> MHYAEAATPAKSAGSAVAKKHLEAKQKIGFVHGIDGTIATIAPAASKVTVPYNTVLEIAVSATNIANALVFNLEKDGSIGVILLDNISEVRSGQDVYATGSLLKIPVGFHMLGKIINPLGKEIPTGLFTKAAPLLDDTKLGLVEEMAPNIVSRQPVNYNLLTGYKVIDTLIPVGRGQRELILGDRQTGKTSIALSTILNQTKVNNEILSKNNVLSVYVSIGQ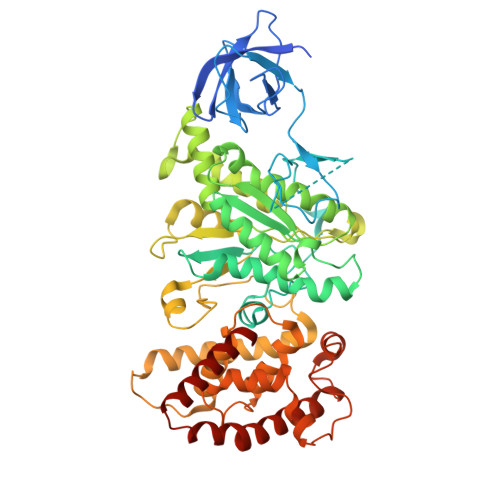RCSNVARIHRLLTEYDAMKYCTIVAATAADPAGLQYLAPYAGTTLGEEFRNSGRHILLVYDDLSKQAVSYRQISLLLRRPPGREAYPGDVFYLHSRLLERSAMMSPQKGSGSLTSLPIVETLSNDVTAYIVTNVISITDGQIYLDAKLFTGGQRPAVNIGLSVSRVGSSAQNKAMKKVGGALKMLMGEYRKMAGEQTSGSQNVSPVMIRGARCLQLFNQKGPSYFMDAIVALYAVTNGYMDDVKLQYSKFYEFLLLNKDLPVLYGQVNNKYFYMYNKNLNYFIRYFGLNHEILEPELKKYIEIHTNLFLDNYQSRMNELKSDEDLVQLKNLLYACKRTV1-[(2~{R},4~{S},5~{R})-5-[[[(2~{R},6~{S})-2-[2,4-bis(oxidanylidene)pyrimidin-1-yl]-6-(hydroxymethyl)morpholin-4-yl]-oxidanyl-phosphinothioyl]oxymethyl]-4-oxidanyl-oxolan-2-yl]-5-methyl-pyrimidine-2,4-dione | C19 H26 N5 O10 P S | 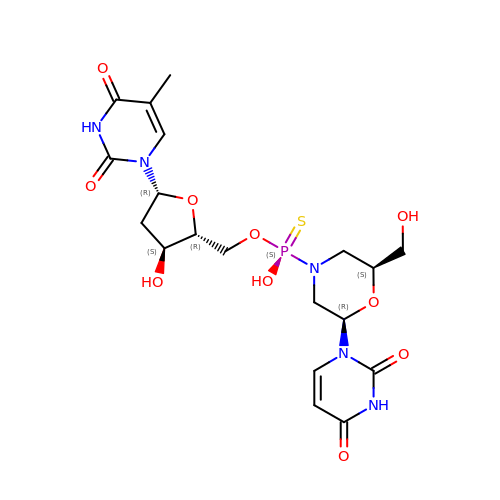JMOYBKKBBMXKAB-OTRGKRLXSA-N> GIAASRLDEIM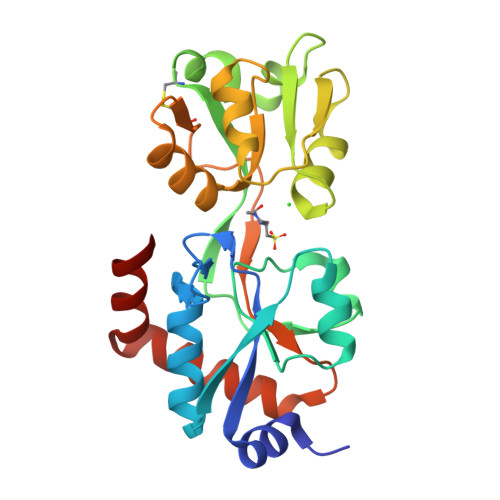QRGTLRVGTTGDYKPFSYRDPDGQFTGFDIDMAESLAKSLGVKVEFVPTTWPTLMDDFQADKFDIAMGGVSVTPERQKKADFSEPYMTDGKTPIVRCEDADKYQTLEQIDRPDVRVVVNPGGTNERFARAHLKQAQITVYPDNVTIFQEIVAGRADVMMTDAVETRYQQKLHPGLCAVHVDKPFTHSEKAYLLPRGDPAFKAYVDQWLHQAMQSGTYQRIFDKWLKL4-[(piperazin-1-yl)methyl]-N-{[4-({[(pyridin-3-yl)methyl]carbamoyl}amino)phenyl]methyl}benzamide 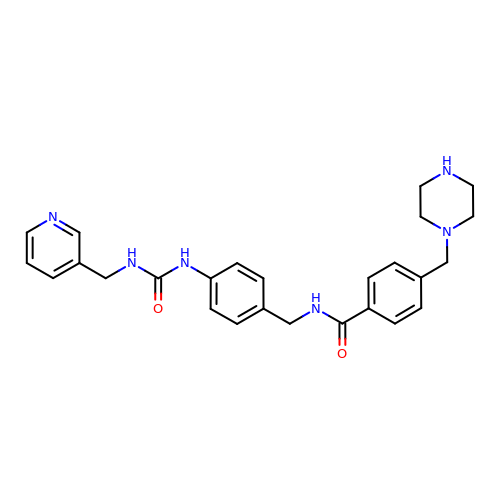| C26 H30 N6 O2 | UPQVXXVUUYBILK-UHFFFAOYSA-N> GALNRKVKNNPDPTIYPVLDWNDIKFQDVIGEGNFGQVLKARIKKDGLRMDAAIKRMKEYASKDDHRDFAGELEVLCKLGHHPNIINLLGACEHRGYLYLAIEYAPHGNLLDFLRKSRVLETDPAFAIANSTASTLSSQQLLHFAADVARGMDYLSQKQFIHRNLAARNILVGENYVAKIADFGLSRGQEVYVKKTMGRLPVRWMAIESLNYSVYTTNSDVWSYGVLLWEIVSLGGTPYCGMTCAELYEKLPQGYRLEKPLNCDDEVYDLMRQCWREKPYERPSFAQILVSLNRMLEERKTYVNTTLYEKFTYAGI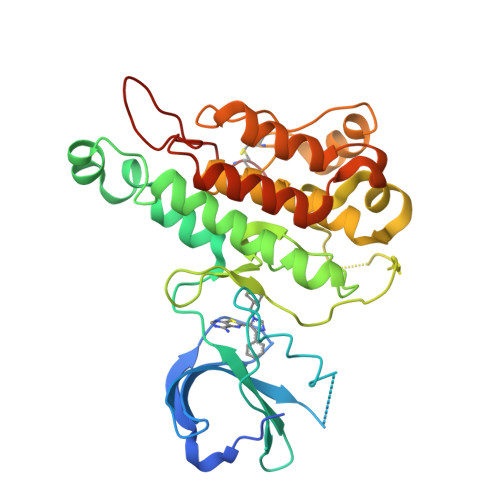DCSAEEAA> MNFSGGGRQE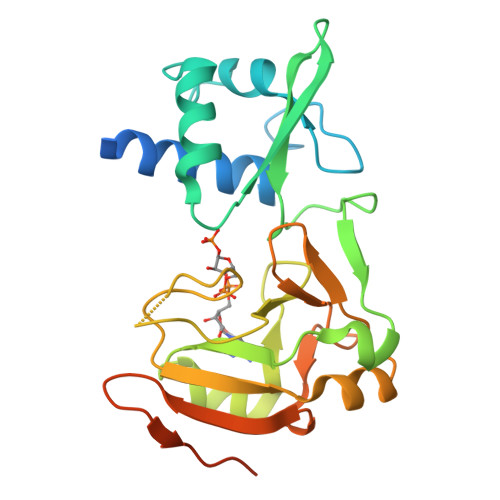AAGSRGRRAPRPREQDRDVQLSKALSYALRHGALKLGLPMGADGFVPLGTLLQLPQFRGFSAEDVQRVVDTNRKQRFALQLGDPSTGLLIRANQGHSLQVPKLELMPLETPQALPPMLVHGTFWKHWPSILLKGLSCQGRTHIHLAPGLPGDPGIISGMRSHCEIAVFIDGPLALADGIPFFRSANGVILTPGNTDGFLLPKYFKEALQLRPTRKPLSLAGDEETECQSSPKHSSRERRRIQQ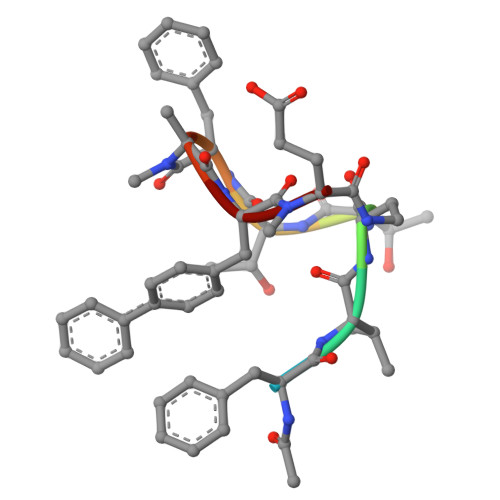> XFVATTFAFX> DTYTGFCIIKEGTKISKSGWEVLSFTTQEASGEGAGNGLAKCLIDGDTETFWHAKWQGGSDPLPYDIVIDMKQNIQIAQVELLPRGRGSNNPIKVVEFAASEDNVNWTPIGRFGFTNQDAALEYYVKSIKARYIR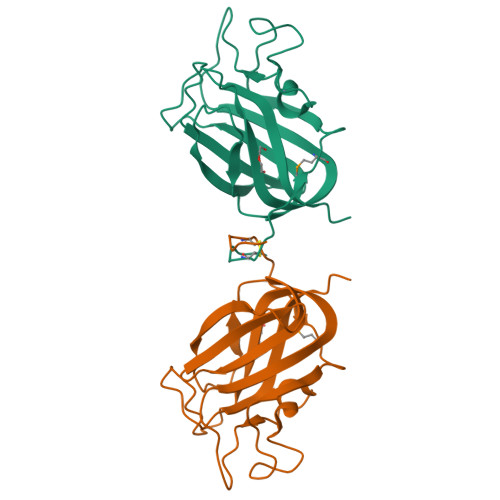LTIPDDGGNSTVAAIRELDVKGTIINLEHHHHHH N-[(3aS,4R,5S,6S,6aS)-4,5,6-trihydroxy-4-(hydroxymethyl)-4,5,6,6a-tetrahydro-3aH-cyclopenta[d][1,3]thiazol-2-yl]-alpha- 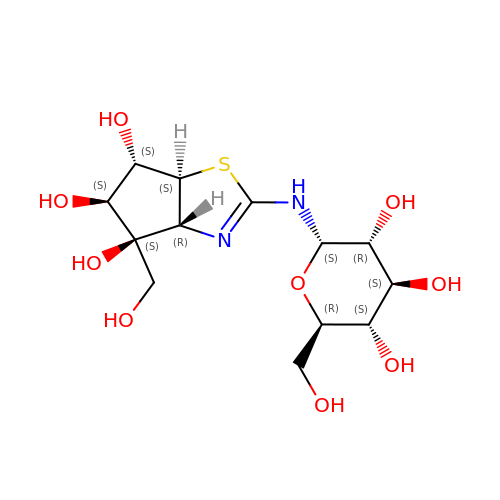D-glucopyranosylamine | C13 H22 N2 O9 S | UISBBVOCYJQFAA-UXTOMXPUSA-N> NNFNYGAYHSLEAIYHEMDNIAADFPDLARRVKIGHSFENRPMYVLKFSTGKGVRRPAVWLNAGIHSREWISQATAIWTARKIVSDYQRDPAITSILEKMDIFLLPVA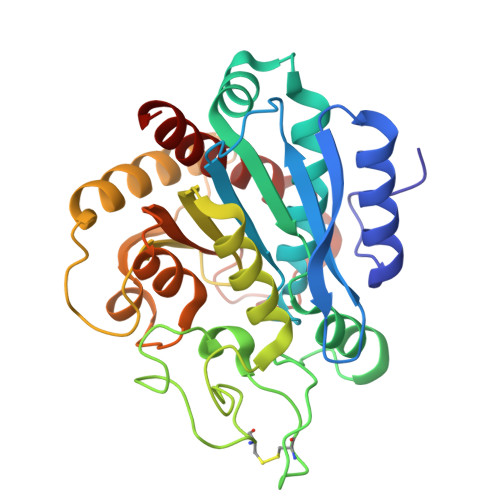NPDGYVYTQTQNRLWRKTRSRNPGSSCIGADPNRNWNASFAGKGASDNPCSEVYHGPHANSEVEVKSVVDFIQKHGNFKGFIDLHSYSQLLMYPYGYSVKKAPDAEELDKVARLAAKALASVSGTEYQVGPTCTTVYPASGSSIDWAYDNGIKFAFTFELRDTGTYGFLLPANQIIPTAEETWLGLKTIMEHVRDNL> GSGCFGYKCDYYKGCCSGYVCSPTWKWCV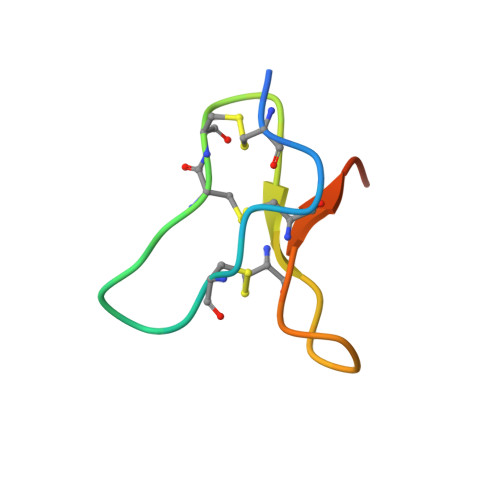RPGPGR> MGSHHHHHHSQDPVQDIEDEASNNVDHDYVYPLPENMVYRFDKSTNILDYLS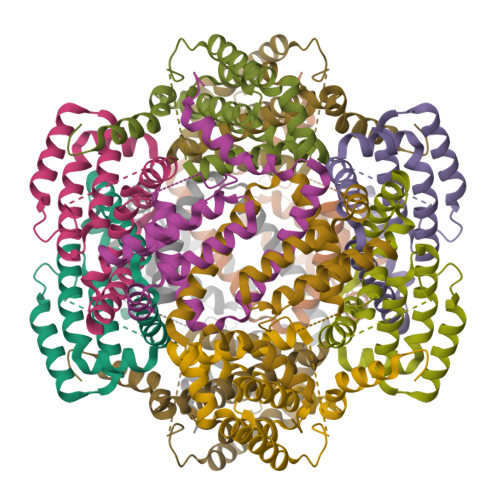TERDHVMMAVRYYMSKQRLDDLYRQLPTKTRSYIDIINIYCDKVSNDYNRDMNIMYDMASTKSFTVYDINNEVNTIMLDNKGLGVRLATISFITELGRRCMNPVKTIKMFTLLSHTICDDCFVDYITDIS>MHHHHHHLPNITILATGGTIAGGGDSATKSNYTVGKVGVENLVNAVPQLKDIANVKGEQVVNIGSQDMNDNVWLTLAKKINTDCDKTDGFVITHGTTTMEETAYFLDLTVKCDKPVVMVGAMRPSTSMSADGPFNLYNAVVTAADKASANRGVLVVMNDTVLDGRDVTTTNTTDVATFKSVNYGPLGYIHNGKIDYQ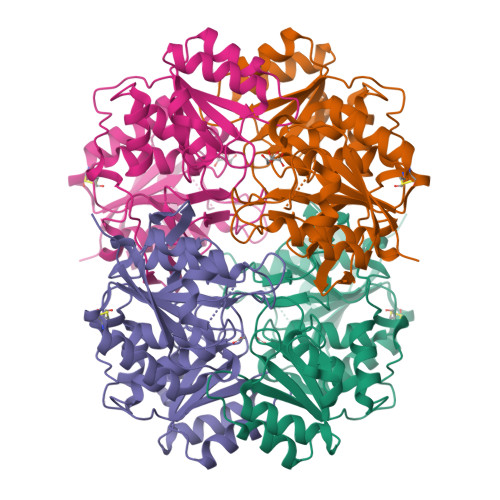RTPARKHTSDTPFDVSKLNELPKVGIVYNYANASDLPAKALVDAGYDGIVSAGVGNGNLYKSVFDTLATAAKTGTAVVRSSRVPTGATTQDAEVDDAKYGFVASGTLNPQKARVLLQLALTQTKDPQQIQQIFNQY[2x]We report the functional characterisation of a modified sugar-binding protein, MsBP, from a marine Synechococcus strain, MITS9220. Ligand screening of MsBP shows a specific affinity for zinc (KD ~ 1.3 μM) and a preference for phosphate-modified sugars, such as fructose-1,6-biphosphate, in the presence of zinc (KD ~ 5.8 μM). The presence of the additional C-terminal subdomain places it unambiguously within sub-cluster D-I, associated with a narrow substrate preference for carbohydrates.

Our crystal structures of apo MsBP (no zinc or substrate-bound) and Zn-MsBP (with zinc-bound) show that the presence of zinc induces structural differences, leading to a partially-closed substrate-binding cavity. The structure of MsBP displayed two chains in the a.s.u. No electron density attributable to a ligand was distinguished in either structure, indicating both proteins were crystallised in ligand-free forms. The intervening binding cleft shows a markedly positive charge, suggestive for orienting a negatively charged substrate. Overall, the structures of MsBP and Zn-MsBP overlay with r.m.s.d. 0.87 Å (Cα atoms), with the most striking difference caused by marked and localised tilting of helix 2, attributable to a lower degree of conformational variability in loop 3. As previously discussed, the general nature of the binding cleft of MsBP is positively charged, which is markedly different from structural relatives that display negatively charged binding cavity, appropriate for interaction with simple sugars.

>[2x]MGSSHHHHHHSSGLVPRGSMRGSHMPEGTLQLWTLQLAPKFNPYMDDVLGSWDKLHPEALVRWTDLPWGSVERKLLAAVFARTAPDVVNLNPPFAANLASKGGLTDLTALLPPGAEQNYLPSVWEAARDPEAGQIAIPWYLTVRLSLVNGDLLRQAGLSRAPRRWDEVPAYARSIRERTGRYGLFVTVVPDDSAELLESFVQMGVSLLDARQRAAFNTPAGRKAFAFWTDLYREGLLPREVVSQGQRRAIELYQSGELALLASGAEFLRSIQTNAPGVAAVTTPQPPLTGSDGTANVALMTLAVPRQSQQAGEAVELALFLTNGTNQARFAREARVLPSSLEALSAIRAELEVEQPSNPAEAQIRDARLLSAETLNTARVLVPATPGVKRLQSIIYTQLQRAMLGQISSDQAVLEAEQQWNRYASARWP N-[2,4-bis(fluoranyl)-3-[2-(3-methoxy-1H-pyrazolo[3,4-b]pyridin-5-yl)ethynyl]phenyl]-3-bromanyl-benzenesulfonamide 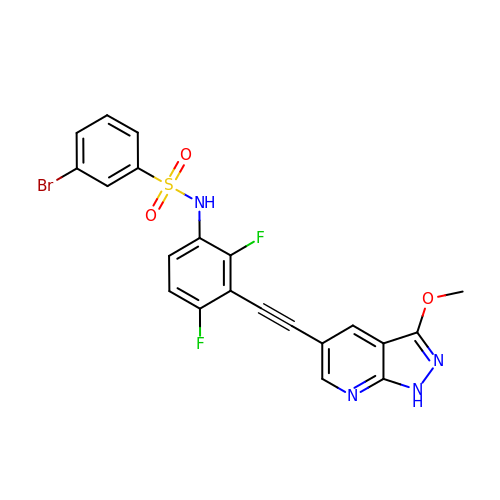| C21 H13 Br F2 N4 O3 S | PJGQKTLXZJMPIM-UHFFFAOYSA-N>[12x]SNAMRLWLIRHGETQANVDGLYSGHAPTPLTARGIEQAQNLHTLLDDVSFDLVLCSELERAQHTARLVLSDRQLPVHIIPELNEMFFGDWEMRHHRDLMQEDAENYSAWCNDWQHAIPTNG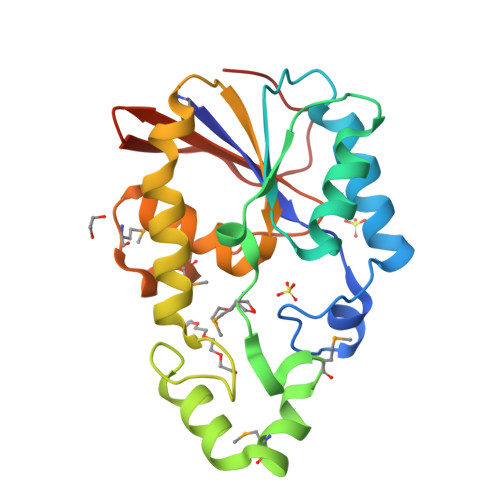EGFQAFSQRVERFIARLSEYQHYQNILIVSHQGVLSLLIARLIGMPAESMWHFRVDQGCWSAIDINQKFATLRVLNSRAIGVENA> MNCKNMDTSYEIINYLTKDELDIDLSQMDKKERYKIWKRLPKCELHCHLDVCFSVDFFLNVIRKYNIQPNMSDEEIIDYYLFSKPGKSLDEFVEKALRLTDIYIDYTVVEDLAKHAVFNKYKEGVVLMEFRYSPSFMSFKHNLDKDLIHEAIVKGLNEAVALLEYKIQVGLLCTGDGGLSHERMKEAAEFCIKHKKDFVGYDHAGHEVDLKPFKDI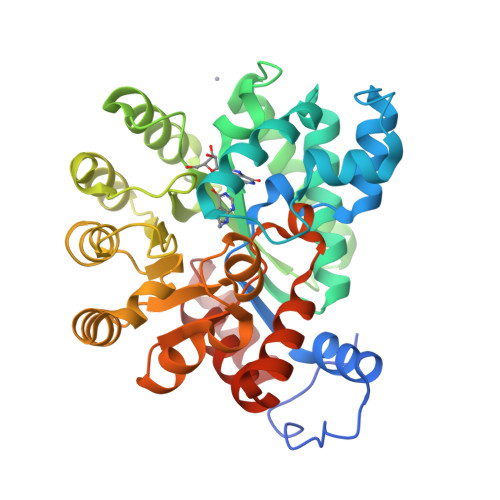FDNIREEGISISVHAGEDVSIPNLNSLYTAINLLHVKRIGHGIRVSESQELIDLVKEKDILLEVCPISNVLLNNVKSMDTHPIRMLYDAGVKVSVNSDDPGMFLTNITDNYEELYTHLNFTLADFMKMNLWAVQKSFVDPDIKNKIISKYF>SIPGQVADQAPLPSLAPMLEKVLPAVVSVRVEGTASQGQKIPEEFKKFFGDDLPDQPAQPFEGLGSGVIINASKGYVLTNNHVINQAQKISIQLNDGREFDAKLIGSDDQSDIALLQIQNPSKLTQIAIADSDKLRVGDFAVAVGNPFGLGQTATSGIVS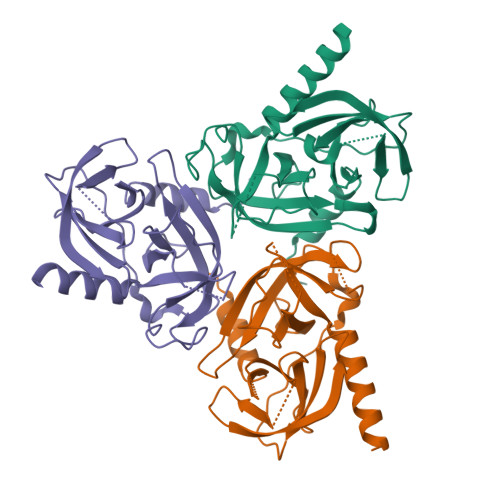ALGRSGLNLEGLENFIQTDASINRGNSGGALLNLNGELIGINTAILAPGGGSVGIGFAIPSNMARTLAQQLIDFGEILEHHHHHH[3x]>[2x]SMSGIALSRLAQERKAWRKDHPFGFVAVPTKNPDGTMNLMNWECAIPGKKGTPWEGGLFKLRMLFKDDYPSSPPKCKFEPPLFHPNVYPSGTVCLSILEEDKDWRPAITIKQILLGIQELLNEPNIQDPAQAEAYTIYC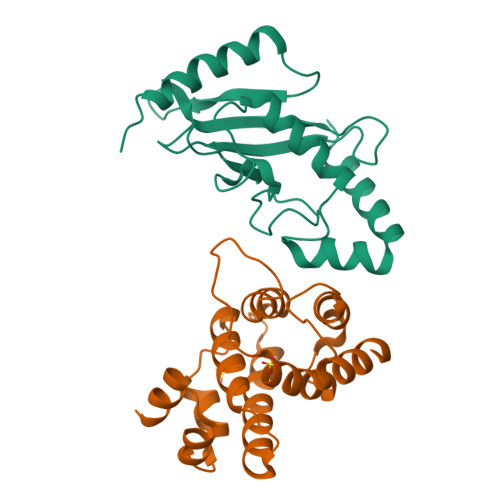QNRVEYEKRVRAQAKKFAPS;>SNSGEPAPVLSSPTPTDLSTFLSFPSPEKLLRLGPKVSVLIVQQTDTSDPEKVVSAFLKVASVFRDDASVKTAVLDAIDALMKKAFSCSSFNSNTFLTRLLIHMGLLKSEDKIKAIPSLHGPLMVLNHVVRQDYFPKALAPLLLAFVTKPNGALETCSFARHNLLQTLYNI[2x]> 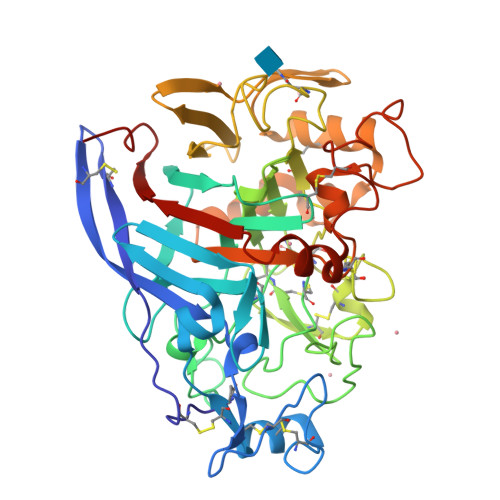QSACTLQSETHPPLTWQKCSSGGTCTQQTGSVVIDANWRWTHATNSSTNCYDGNTWSSTLCPDNETCAKNCCLDGAAYASTYGVTTSGNSLSIGFVTQSAQKNVGARLYLMASDTTYQEFTLLGNEFSFDVDVSQLPCGLNGALYFVSMDADGGVSKYPTNTAGAKYGTGYCDSQCPRDLKFINGQANVEGWEPSSNNANTGIGGHGSCCSEMDIWEANSISEALTPHPCTTVGQEICEGDGCGGCYSDNRYGGTCDPDGCDWNPYRLGNTSFYGPGSSFTLDTTKKLTVVTQFETSGAINRYYVQNGVTFQQPNAELGSYSGNELNDDYCTAEEAEFGGSSFSDKGGLTQFKKATSGGMVLVMSLWDDYCANMLWLDSTYPTNETSSTPGAVRGSCSTSSGVPAQVESQSPNAKVTFSNIKFGPIGSTGNP> KDQIPIILIHGSGGNASSLDKMADQLMNEYRSSNEALTMTVNSEGKIKFEGKLTKDAKRPIIKFGFEQNQATPDDWSKWLKIAMEDLKSRYGFTQMDGVGHSNGGLALTYYAEDYAGDKTVPTLRKLVAIGSPFNDLDPNDNGMDLSFKKLPNSTPQMDYFIKNQTEVSPDLEVLAIAGELSEDNPT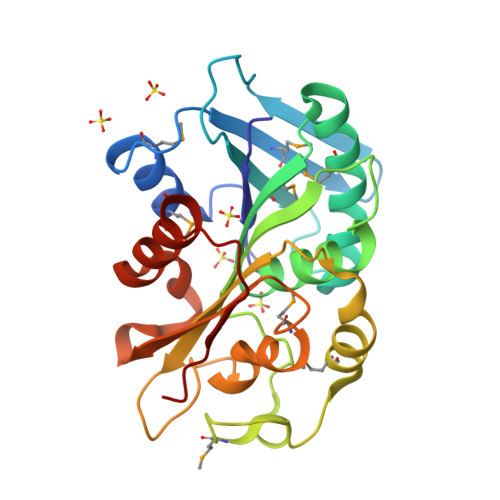DGIVPTISSLATRLFMPGSAKAYIEDIQVGEDAVHQTLHETPKSIEKTYWFLEKFKTDETVIQLDYK Thioredoxins (TRX) are small globular proteins of about 100–110 residues, which are conserved in all living organisms. They participate in multiple critical redox-reactions via the reversible oxidation of the active site CXXC catalytic motif1. Two TRX forms were described in Escherichia coli, Trx1 and Trx22. The former, called EcTRX throughout this work, is a widely used experimental model for investigating the molecular basis of protein stability, folding and function.

The L94A mutation was introduced to disrupt the van der Waals interactions between Leu94 and the Leu99 residue of the CTH, with a concomitant destabilization of the global structure through intramolecular packing defects. In the crystal structure of wild-type EcTRX, two small cavities of 70 and 50 Å2 of internal area are localized near Leu94, which coalesce in a larger cavity of 183 Å2 in the L94A mutant structure. This effect approaches what can be expected from pruning the side-chain to Cβ in the wild-type structure. A decrease of the distance between loop elements centered in residues 20 and 83 is observed in this mutant in a similar manner as described for the N106A variant. We determined in this work the three-dimensional structure of three full-length variants in which the point mutations occur in the CTH (E101G, N106A and L107A), and one additional variant (L94A) where a substitution is located in the loop connecting β5-strand and CTH, using X-ray diffraction. The four EcTRX mutants were crystallized in the oxidized form, and numerous protein-metal interactions were observed as a result of the Cu(II)-salt added for crystallization, as it was previously observed for the wild-type variant. Notably, the four variants crystallized in different crystal systems, comprising monoclinic, triclinic, orthorhombic and trigonal space groups, for L94A, E101G, N106A and L107A respectively. As expected from solution experiments, the global structures of the four variants are mainly unchanged compared to wild-type EcTRX, with main-chain root-mean-square deviation of atomic position (RMSD) differences of 0.59, 0.48, 0.62 and 0.48 Å for L94A, E101G, N106A and L107A, respectively. We found that global stability of the variants is progressively altered from 8.1 (wild-type), 7.8 (N106A), 7.4 (L94A), 7.2 (E101G) to 5.8 kcal mol−1 (L107A). Previous results of our group showed that the specific activity measured by using the non-natural substrate DiFTC-insulin is 80, 95, 100, 108 and 175% for L94A, L107A, wild-type, N106A and E101G, respectively. For variant L94A, the drop was a 1:1 mix of protein (10 mg/ml) and reservoir solution (100 mM sodium acetate, 4 mM CuSO4, 18% ethanol, pH 4.6).

> MSDKIIHLTDDSFDTDVLKADGAILVDFWAEWCGPCKMIAPILDEIADEYQGKLTVAKLNIDQNPGTAPKYGIRGIPTLLLFKNGEVAATKVGAASKGQLKEFLDANLA> LGSSNDNIELVDFQNIMFYGDAEVGDNQQPFTFILDTGSANLWVPSVKCTTAGCLTKHLYDSSKSRTYEKDGTKVEMNYVSGTVSGFFSKDLVTVGNLSLPYKFIEVIDTNGFEPTYTASTFDGILG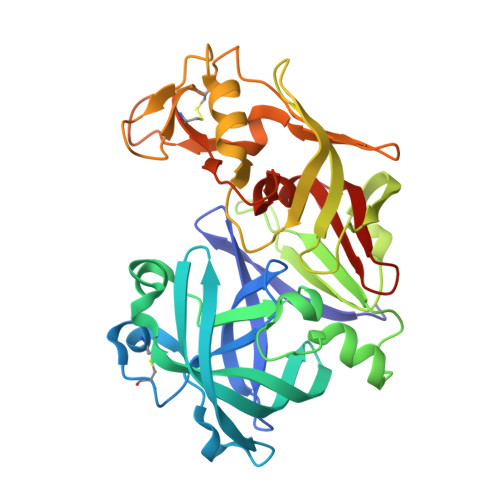LGWKDLSIGSVDPIVVELKNQNKIENALFTFYLPVHDKHTGFLTIGGIEERFYEGPLTYEKLNHDLYWQITLDAHVGNIMLEKANCIVDSGTSAITVPTDFLNKMLQNLDVIKVPFLPFYVTLCNNSKLPTFEFTSENGKYTLEPEYYLQHIEDVGPGLCMLNIIGLDFPVPTFILGDPFMRKYFTVFDYDNHSVGIALAKKNL>[8x]GSGLNIKENDLPGIGKKFEIETRSHEKMTIIIHDDGRREIYRFNDRDPDELLSNISLDDSEARQIAAILGGMVYKPQALESIEMAFSDLIIE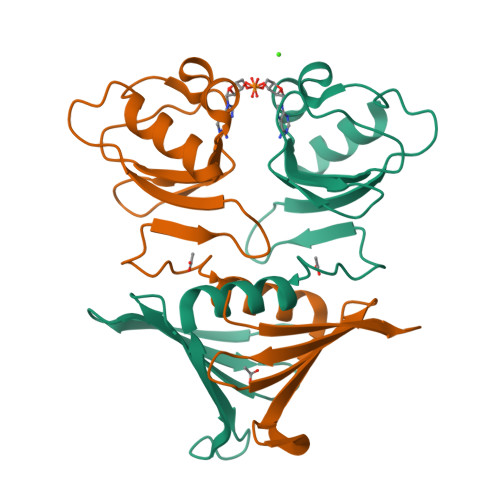WFKVEKGAKSIGRTLGELDVRQNYDVTVIAIIKHNQEKLLNPGADSIIEENDTLVLSGERKHLKKLIHDFLSGEGV>ANQEKKLGEYSKKAAMKPKPLSVLKSLEEKYVAVMKKLQFDTFEMVSEDEDGKLGFKVNYHYMSQVKNANDANSAARARRLAQEAVTLSTSLPLSSSSSVFVRCDEERLDIMKVLITGPADTPYANGCFEFDVYFPQDYPSSPPLVNLETTGGHSVRFNPNLYNDGKVCLSILNTWHGRPEEKWNPQTSSFLQVLVSVQSLILVAEPYFNEPGYERSRGTPSGTQSSREYDGNIRQATVKWAMLEQIRNPSPCFKEVIHKHFYLKRVEIMAQCEEWIADIQQYSSDKRVGRTMSHHAAALKR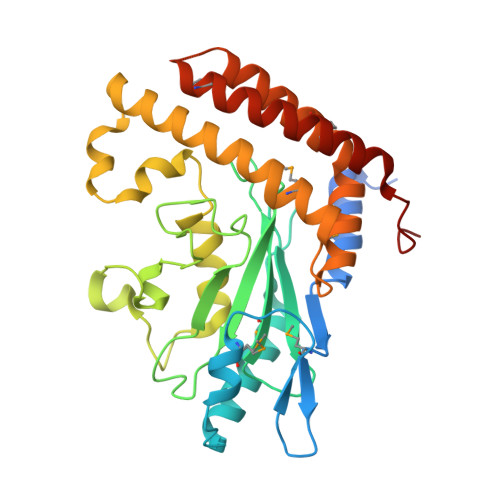HTAQLREELLKLPCPEGLDPD[2x]>SSHHHHHHMSGENLYFQGASAAIVTDTGGVDDKSFNQSAWEGLQAWGKEHNLSKDNGFTYFQSTSEADYANNLQQAAGSYNLIFGVGFALNNAVKDAAKEHTDLNYVLIDDVIKDQKNVASVTFADNESGYLAGVAAAKTTKTKQVGFVGGIESEVISRFEAGFKAGVASVDPSIKVQVDYAGSFGDAAKGKTIAAAQYAAGADIVYQVAGGTGAGVFAEAKSLNESRPENEKVWVIGVDRDQEAEGKYTSKDGKESNFVLVSTLKQVGTTVKDISNKAERGEFPGGQVIV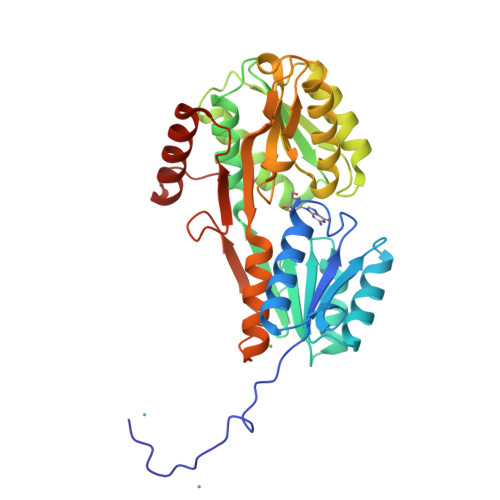YSLKDKGVDLAVTNLSEEGKKAVEDAKAKILDGSVKVPEK[4x]> N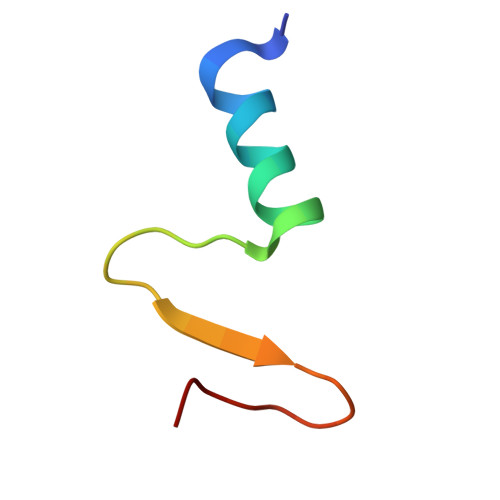GGQEALEERARNELSMTRPGETFYRLVPDASKRA>[4x]MSYQSTIVPVELHSFEDAQVIGGAFRDGDAVVFDMSLLSREEARRIVDFAAGLCFALRGKMQKIDSVTFAVVPE;>[4x]DDLDVPSFLQ

At the cell division site, FtsZ protofilaments form a highly dynamic, membrane-bound structure, the Z-ring, which serves as a scaffold for the recruitment of the extra-cytoplasmic cell wall biosynthetic machinery. Here we investigate the physiological function of Corynebacterium glutamicum SepF, the only cell division-associated protein from Actinobacteria known to interact with the conserved C-terminal tail of FtsZ. Our structural data revealed the FtsZ-binding pocket, defining the SepF homodimer as the functional unit, and suggesting a reversible β-sheet-mediated oligomerization interface possibly regulated via an alpha helical switch. We found that FtsZ filaments and lipid membranes have opposing effects on SepF polymerization, pointing to a complex dynamic role of the protein at the division site, involving FtsZ bundling, Z-ring tethering and membrane reshaping activities that are needed for proper Z-ring assembly and function.

To further investigate this hypothesis, we removed the helix and crystallized the resulting SepFΔML,Δα3 construct alone and in complex with FtsZCTD. Despite a different crystal packing, the two structures did show a dimer-dimer association mediated by the opposing β-sheets in the crystal, generating linear SepF polymers similar to those observed for the B. subtilis homolog. These observations demonstrate that the β-sheet is indeed prone to self-interaction in solution and suggest that the amphipathic helix α3 might regulate SepF polymerization. When the same experiment was carried out with SepFΔα3, lacking the regulatory C-terminal helix, polymerization and vesicle tubulation were also seen but could only be partially reversed after addition of the FtsZCTD peptide.>[2x]MSERTGTQPLGVQGLTEEQRMMIRELMDAQMKTFDTTFSHFKNFRLPGVLSSGCELPESLQAPSREEAAKWSQVRKDLCSLKVSLQLRGEDGSVWNYKPPADSGGKEIFSLLPHMADMSTYMFKGIISFAKVISYFRDLPIEDQISLLKGAAFELCQLRFNTVFNAETGTWECGRLSYCLEDTAGGFQQLLLEPMLKFHYMLKKLQLHEEEYVLMQAISLFSPDRPGVLQHRVVDQLQEQFAITLKSYIECNRPQPAHRFLFLKIMAMLTELRSINAQHTQRLLRIQDIHPFATPLMQELFGITGSSSSGGTCPSSHSSLTERHKILHRLLQEGSPSAAA

In mammals, pregnane X receptor (PXR) is a major regulator of the expression of drug metabolism and xenobiotic detoxification genes. In mammals, PXR is a major transcription factor for regulating the expression of phase I–III drug metabolising/xenobiotic detoxifying genes. Nomilin is a naturally-occurring compound in citrus fruits such as lemons, grapefruits, oranges as well as in tangerine seed and peel. Here, we show that nomilin is a PXR agonist, and may extend lifespan and healthspan in C. elegans and mice via NHR-regulated detoxification functions, and induce the common transcriptome markers seen in the liver of mice in response to most lifespan-extending interventions.

To further confirm the direct binding between nomilin and hPXR, and discover more information on its structure and activation mechanism, we expressed the ligand-binding domian (LBD) domain of hPXR (residues 130–432) fused with residues 676–700 of nuclear receptor coactivator 1 (NCOA1676–700) at the C-terminal as a co-activator peptide. The purified hPXRLBD-NCOA1676–700 (hPXR chimera hereafter) was co-crystallised with nomilin and the structure of the protein-drug complex was determined at a resolution of 2.1 Å, allowing a detailed observation of the drug-target interaction. The hPXR chimera forms a homodimer in the purification and crystal structure, as previously reported. The dimeric hPXR forms an interface via the β1' strand of the characteristic antiparallel β-sheet. A region of non-proteinaceous electron density was identified in the Fo-Fc map of the LBDs of each of the hPXR protomers, and the molecular framework of nomilin fit the electron density very well. The electron density in protomer A was refined with better continuity than that in protomer B. The binding of nomilin in the hPXR chimera was majorly mediated by the hydrogen bonds formed by two carbonyl oxygens with S247 and Q285, as well as the strong hydrophobic interaction among the backbone carbons of nomilin, and the cavity formed by a series of hydrophobic residues including M243, W299, I414 and M425. Two methionine residues, M243 and M425, closely contact both nomilin and rifampicin in their crystal structures, respectively. In addition, one of the structural differences between hPXR bound with nomilin and rifampicin is the helix formed by amino acids 193–209, which is well-refined in our structure and previously reported structures of hPXR in complex with SR12813, clotrimazole, and hyperforin, but absent in the structure of hPXR-rifampicin complex. However, S247A/R, M425A/Q and W299R completely blocked the activity of nomilin, indicating that these amino acid residues are critical for nomilin-dependent hPXR activation.>[2x]GPGSMSNSYEGCGDLTIFVAVALNKVIGHKNQIPWPHITHDFRFLRNGTTYIPPEVLSKNPDIQNVVIFGRKTYESIPKASLPLKNRINVILSRTVKEVPGCLVYEDLSTAIRDLRANVPHNKIFILGGSFLYKEVLDNGLCDKIYLTRLNKEYPGDTYFPDIPDTFEITAISPTFSTDFVSYDFVIYERKDCKTVFPDPPFDQLLMTGTDISVPKPKYVACPGVRIRNHEEFQYLDILADVLSHGVLKPNRTGTDAYSKFGYQMRFDLSRSFPLLTTKKVALRSIIEELLWFIKGSTNGNDLLAKNVRIWELNGRRDFLDKNGFTDREEHDLGPIYGFQWRHFGAEYLDMHADYTGKGIDQLAEIINRIKTNPNDRRLIVCSWNVSDLKKMALPPCHCFFQFYVSDNKLSCMMHQRSCDLGLGVPFNIASYSILTAMVAQVCGLGLGEFVHNLADAHIYVDHVDAVTTQIARIPHPFPRLRLNPDIRNIEDFTIDDIVVEDYVSHPPIPMAMSA

In this work, we describe the structural features of dihydrofolate reductase-thymidylate synthase from B. bovis (BbDHFR-TS), the causative agent of babesiosis in cattle. BbDHFR-TS is a homodimer that exhibits the classical dimeric interface seen in other structures of ThyA thymidylate synthase and bifunctional DHFR-TS enzymes. This 511-residue, 58.2 kDa bifunctional enzyme consists of a di­hydrofolate reductase (DHFR) subunit at the N-terminus and a thymidylate synthase (TS) subunit at the C-terminus connected by a linker. BbDHFR-TS is an obligate dimer, with two arginine side chains (Arg373′ and Arg374′) from a flexible loop in one protomer making contact with the terminal phosphate of the substrate dUMP in the opposite protomer.

Pemetrexed and raltitrexed are folate analogs designed as antitumour agents and currently approved for use in some countries for treatment of cancer. The two complex structures of BbDHFR-TS have two ligands bound to each subunit of each protomer in the asymmetric unit. The pteroyl-like groups of pemetrexed and raltitrexed are parallel to the uracil ring of dUMP when bound, mimicking the pteridine ring of the native cofactor mTHF. Although the ϕ angle of the C-terminal Ala511 in one protomer of the raltitrexed complex is rotated by approximately 30° relative to the other, this has no effect on the virtually identical binding modes of raltitrexed in both TS subunits in a single crystal structure. Both drug molecules are also observed in the DHFR subunit but appear to bind this substrate pocket with different geometries. The bound conformation of pemetrexed is virtually identical in both DHFR protomers but differs slightly from that of raltitrexed, which itself has two different binding modes for its glutamate tail. However, the para-substitution pattern of benzamide in pemetrexed allows the formation of a salt bridge between the α-COOH of its glutamate tail and the Arg83 side chain. This is in contrast to the 2,5-­disubstituted thiophene ring of raltitrexed with no salt bridge to Arg83. The five-membered ring of raltitrexed causes a >90° rotation and a 6.8 Å translation of its α-COOH group relative to pemetrexed. Moreover, the glutamate tail of raltitrexed is shifted between protomers of DHFR in the same crystal, with both making hydrogen bonds to Arg42 but only one contacting the N∊ atom of His33. The loss of salt bridge and distinct binding modes of raltitrexed thus provide a structural basis for its lower DHFR affinity relative to pemetrexed, independent of the reduced chemical affinity associated with its C2-methylpteroyl scaffold.> MEFWRLVVRPTRRANLVAKLMRDLESGHFAAPKALDVLTQYRTEQLSYSLTGIPRVTLPEKPLIRAFLQKYPEARAEPVALDSFTPPLARQFAQRQ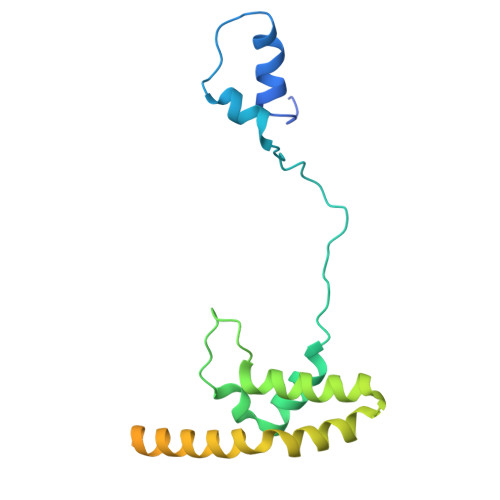LQLMQAGAAREQAFTQAEQELAGRLQALRSRLLGSAATALSEGAQAAVPGPAASGVRGMVELLQQEEQEALDAGLEALASSAQQQQQQLSANSR>MFEVKMGSKMCMNASCGTTSTVEWKKGWPLRSGLLADLCYRCGSAYESSLFCEQFHKDQSGWRECYLCSK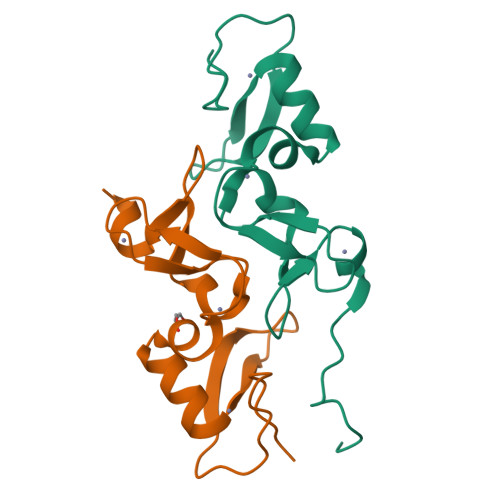RLHCGCIASKVTIELMDYGGVGCSTCACCHQLNLNTRGEN[4x]>[6x]GGNDRVRNLQSEVEGVKNIMTQNVERILARGENLEHLRNKTEDLEATSEHFKTTSQKVARKFWWKNVK;>HTTEA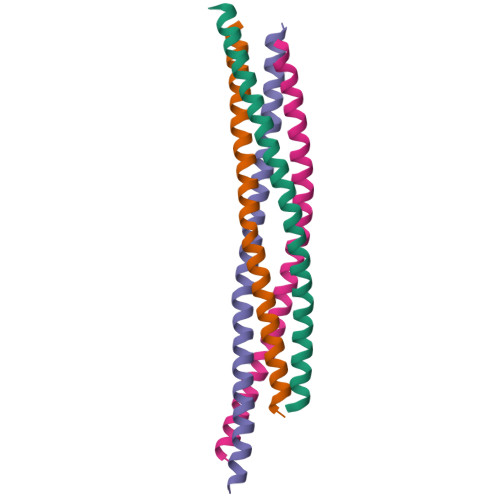EASSQSLTQIYALPEIPQDQNAAESWETLEADLIELSQLVTDFSLLVNSQQEKIDSIADHVNSAAVNVEEGTKNLGKAAKYK[6x];>[6x]DRQQYLRQEVLRRAEATAASTSRSLALMYESEKVGVASSEELARQRGVLERTEKMVDKMDQDLKISQKHINSIKSVFGGLVNYFKSKPVET;>KNPHLRAYHQKIDSNLDELSMGLGRLKDIALGMQTEIEEQDDILDRLTTKVDKLDVNIKSTERKVRQL[6x]>[4x]MTQMLTRPDVDLVNGMFYADGGAREAYRWMRANEPVFRDRNGLAAATTYQAVLDAERNPELFSSTGGIRPDQPGMPYMIDMDDPQHLLRRKLVNAGFTRKRVMDKVDSIGRLCDTLIDAVCERGECDFVRDIAAPLPMAVIGDMLGVLPTERDMLLKWSDDLVCGLSSHVDEAAIQKLMDTFAAYTEFTKDVITKRRAEPTDDLFSVLVNSEVEGQRMSDDEIVFETLLILIGGDETT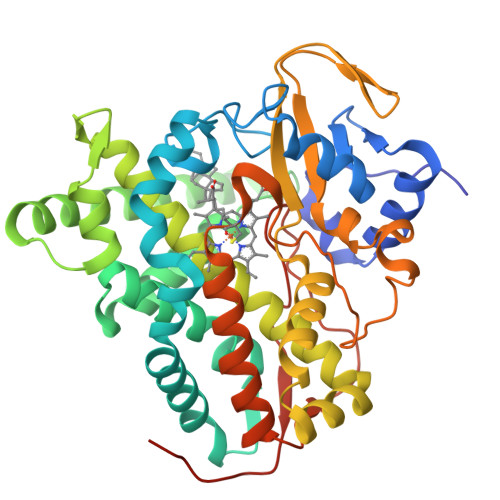RHTLSGGTEQLLRHRDQWDALVADVDLLPGAIEEMLRWTSPVKNMCRTLTADTVFHGTELRAGEKIMLMFESANFDESVFGDPDNFRIDRNPNSHVAFGFGTHFCLGNQLARLELRLMTERVLRRLPDLRLADDAPVPLRPANFVSGPESMPVVFTPSAPVLAHHHHHH> MGEPQQVSALPPPPMQYIKEYTDENIQEGLAPKPPPPIKDSYMMFGNQFQCDDLIIRPLESQGIERLHPMQFDHKKELRKLNMSILINFLDLLDILIRSPGSIKREEKLEDLKLLFVHVHHLINEY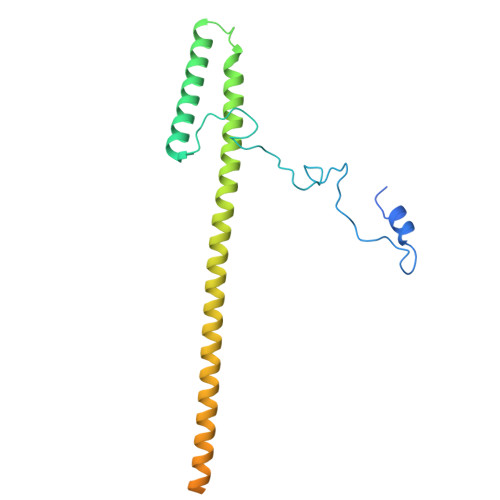RPHQARETLRVMMEVQKRQRLETAERFQKHLERVIEMIQNCLASLPDDLPHSEAGMRVKTEPMDADDSNNCTGQNEHQRENSGHRRDQIIEKDAALCVLIDEMNERP> GMKVTFLGHAVVLIEGKKNIIIDPFISGNPVCPVKLEGLPKIDYILVTHGHGDHLGDAVEIAKKNDATVISNYEICHYLGKKGVKTHAMHIGGSYLFDFGRVKMTPAVHGSGILDGDSMIYGGNPSGFL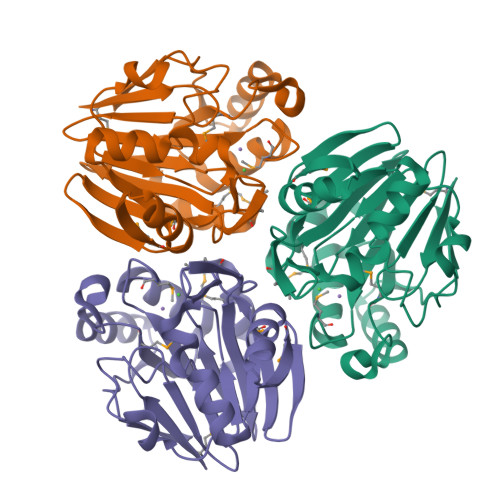ITIEGKKIYHAGDTGLTREMELLAEENVDVAFLPIGGNFVMDVEDAVRAAVMIKPKKVVPMHYGTWELIFADVELFKKKVEEKGVECVILEPGESLEL> GPYKYITEDKYLQTNFYSANQKENVNLNTLDSKSNNSKTITSEERPLSETEQNYVSSTPEPSTPEKVLEKHNKDLDNDPNISQFILNFVNRPERDKLFGSPVAFSKKVLGSNPSSGKEVALTFDDGPFPIYTEKYVDILKS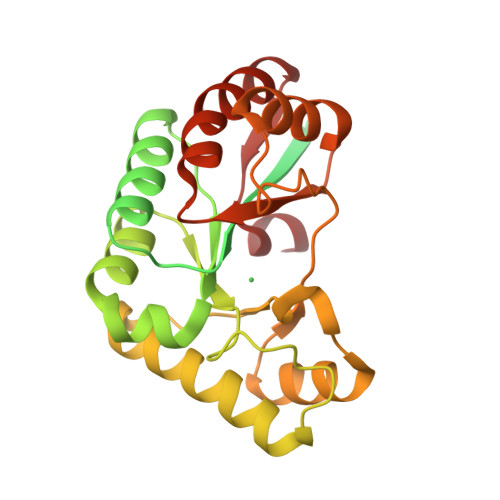MDVKATFFVIGKHAEKHPELLKYIVENGNEIGLHSYSHFNMKKLKPEKMVEELYKTQQIIVEATGIKPTLFRPPFGAYNSTLIEISNALGLKVVLWNVDPDDWRNPSVESVVNRVLSHTRDGSIILMHEGKPSTLAALPQIIKKLKEEGYKFVTVSELLEKRD>[2x]GSHMAIVLGRNQYGKAEVRVFRVYRDTPRHEVRDLNVWTALRGDFTDAHVTGDQSHVLPTDTQKNTVYALAKKEGIRAIEDFALTLGDHFLRQVPAATGARIAIEEYAWDRIDVDGTGHDHGFVRRGQGTRTTVVTVEGRGDERRAWVLSGISDLIIAKTTGSEFHGFLKDEYTTLEETHDRILATSLHTRWRYLTTDVDWDKTFASVRSILLRQFATVHSLAL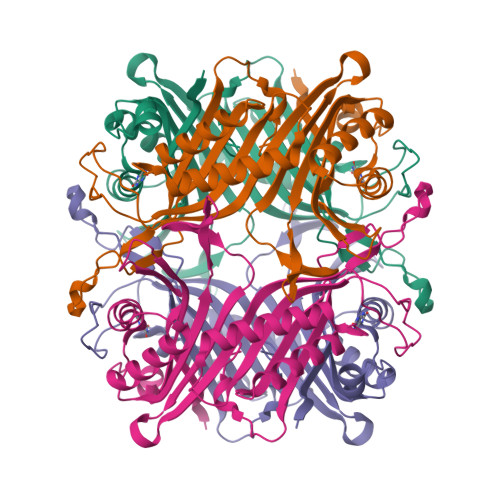QQTLYAMGSAVLEAHPEIAEIRLSAPNKHHFLVDLQPFGLDNPGEVFYASDRPYGLIEASVVRDDVPEAPEAWLATPGFC> MRQVWFSWIVGLFLCFFNVSSAAQYEPPATWENVDYKRTIDVSNAYISETIEITIKNIASEPATEYFTAFESGIFSKVSFFSAYFTNEATFLNSQLLANSTTAPGDDGESEIRYGIIQFPNAISPQEEVSLVIKSFYNTVGIPYPEHVGMSEEQHLLWETNRLPLSAYDTKKASFTLIGSSSFEEYHPPNDESLLGKANGNSFEFGPWEDIPRFSSNETLAIVYSHNAPLNQVVNLRRDIWLSHWASTIQFEEYYELTNKAAKLSKGFSRLELMKQIQTQNMRQTHFVTVLDMLLPEGATDHYFTDLVGLVSTSHAERDHFFIRPRFPIFGGWNYNFTVGWTNKLSDFLHVSSGSDEKFVASIPILNGPPDTVYDNVELSVFLPEGAEIFDIDSPVPFTNVSIETQKSYFDLNKGHVKLTFSYRNLISQVANGQVLIKYDYPKSSFFKKPLSIACYIFTALMGVFVLKTLNMNVTN;> MAKAPKANTPKVTSTSSAVLTDFQETFKTSKRAYFAQIEKYPKLKLIDTFCFFLVLLGVIQCTFIILIRDNFPFNAFLAGFIICVGQFVLLMSLRLQLCNSFPGISKNRAFAEFIVASLILHFVCLHFIN;> MNWLFLVSLVFFCGVSTHPALAMSSNRLLKLANKSPKKIIPLKDSSFENILAPPHENAYIVALFTATAPEIGCSLCLELESEYDTIVASWFDDHPDAKSSNSDTSIFFTKVNLEDPSKTIPKAFQFFQLNNVPRLFIFKPNSPSILDHSVISISTDTGSERMKQIIQAIKQFSQVNDFSLHLPMDWTPIITSTIITFITVLLFKKQSKLMFSIISSRIIWATLSTFFIICMISAYMFNQIRNTQLAGVGPKGEVMYFLPNEFQHQFAIETQVMVLIYGTLAALVVVLVKGIQFLRSHLYPETKKAYFIDAILASFCALFIYVFFAALTTVFTIKSPAYPFPLLRLSAPFK;> MISDEQLNSLAITFGIVMMTLIVIYHAVDSTMSPKN;> MTYEQLYKEFHSSKSFQPFIHLDTQPKFAICGLIVTLAVLSSALFAVGSKSSYIKKLFFYTILSVIGSLFAGLTTVFASNSFGVYV;> MGSDRSCVLSVFQTILKLVIFVAIFGAAISSRLFAVIKFESIIHEFDPWFNYRATKYLVNNSFYKFLNWFDDRTWYPLGRVTGGTLYPGLMTTSAFIWHALRNWLGLPIDIRNVCVLFAPLFSGVTAWATYEFTKEIKDASAGLLAAGFIAIVPGYISRSVAGSYDNEAIAITLLMVTFMFWIKAQKTGSIMHATCAALFYFYMVSAWGGYVFITNLIPLHVFLLILMGRYSSKLYSAYTTWYAIGTVASMQIPFVGFLPIRSNDHMAALGVFGLIQIVAFGDFVKGQISTAKFKVIMMVSLFLILVLGVVGLSALTYMGLIAPWTGRFYSLWDTNYAKIHIPIIASVSEHQPVSWPAFFFDTHFLIWLFPAGVFLLFLDLKDEHVFVIAYSVLCSYFAGVMVRLMLTLTPVICVSAAVALSKIFDIYLDFKTSDRKYAIKPAALLAKLIVSGSFIFYLYLFVFHSTWVTRTAYSSPSVVLPSQTPDGKLALIDDFREAYYWLRMNSDEDSKVAAWWDYGYQIGGMADRTTLVDNNTWNNTHIAIVGKAMASPEEKSYEILKEHDVDYVLVIFGGLIGFGGDDINKFLWMIRISEGIWPEEIKERDFYTAEGEYRVDARASETMRNSLLYKMSYKDFPQLFNGGQATDRVRQQMITPLDVPPLDYFDEVFTSENWMVRIYQLKKDDAQGRTLRDVGELTRSSTKTRRSIKRPELGLRV;> MRTDWNFFFCILLQAIFVVGTQTSRTLVLYDQSTEPLEEYSVYLKDLEQRNYKLEYLDINSTSTTVDLYDKEQRLFDNIIVFPTKGGKNLARQIPVKQLIKFFENEGNILCMSSPGAVPNTIRLFLNELGIYPSPKGHVIRDYFSPSSEELVVSSNHLLNKYVY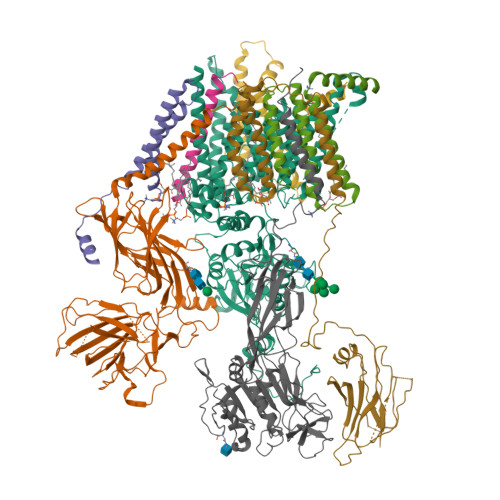NARKSEDFVFGESSAALLENREQIVPILNAPRTSFTESKGKCNSWTSGSQGFLVVGFQNLNNARLVWIGSSDFLKNKNQDSNQEFAKELLKWTFNEKSVIKSVHAVHSHADGTSYDEEPYKIKDKVIYSVGFSEWNGEEWLPHIADDIQFELRQVDPYYRLTLSPSGNDSETQYYTTGEFILPDRHGVFTFLTDYRKIGLSFTTDKDVKAIRHLANDEYPRSWEISNSWVYISAICGVIVAWIFFVVSFVTTSSVGKKLETFKKTN;> MQFFKTLAALVSCISFVLAYVAQDVHVSFPSTAGKSRVMIGKVEPRIGIDETVPTTITVEDPNEVIQVNFAIESTNKPFQNTLLIGLPNKNLEMAFEPEIKDNGKLSMYKYRIDLAKLDAALLQEASRSPEPIKATLILASSTAKPKENLFREILQLNLNFDVDHSDSSLVDKFGIKPEIHHIFHAEPKRVAKPIAVIFVLIIFITILSLIVTWLNSCAAAFNNIPTGVTAVYFLGFIATIVGFEVIFARYYLGTSIFETLFSSLYLGAPGLLTSTKFLRSFGQTI> GMVHYYRLSLKSRQKAPKIVNSKYN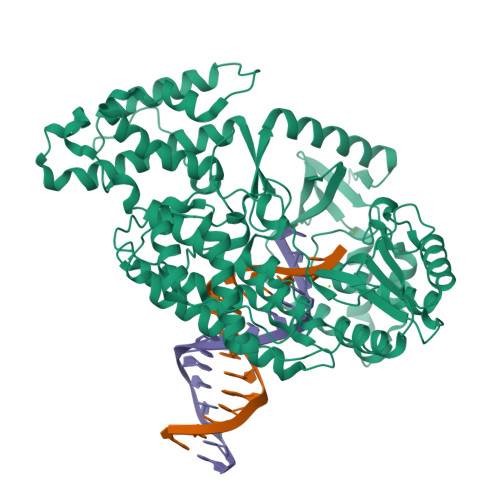SILNIALKNFRLCKKHKTKKPVQILALLQEIIPKSYFGTTTNLKRFYKVVEKILTQSSFECIHLSVLHKCYDYDAIPWLQNVEPNLRPKLLLKHNLFLLDNIVKPIIAFYYKPIKTLNGHEIKFIRKEEYISFESKVFHKLKKMKYLVEVQDEVKPRGVLNIIPKQDNFRAIVSIFPDSARKPFFKLLTSKIYKVLEEKYKTSGSLYTCWSEFTQKTQGQIYGIKVDIRDAYGNVKIPVLCKLIQSIPTHLLDSEKKNFIVDHISNQFVAFRRKIYKWNHGLLQGDPLSGCLCELYMAFMDRLYFSNLDKDAFIHRTVDDYFFCSPHPHKVYDFELLIKGVYQVNPTKTRTNLPTHRHPQDEIPYCGKIFNLTTRQVRTLYKLPPNYEIRHKFKLWNFNNQISDDNPARFLQKAMDFPFICNSFTKFEFNTVFNDQRTVFANFYDAMICVAYKFDAAMMALRTSFLVNDFGFIWLVLSSTVRAYASRAFKKIVTYKGGKYRKVTFQCLKSIAWRAFLAVLKRRTEIYKGLIDRIKSREKLTMKFHDGEVDASYFCKLPEKFRFVKINRKASI>XGELKAIAQELKAIAKELKAIAWEH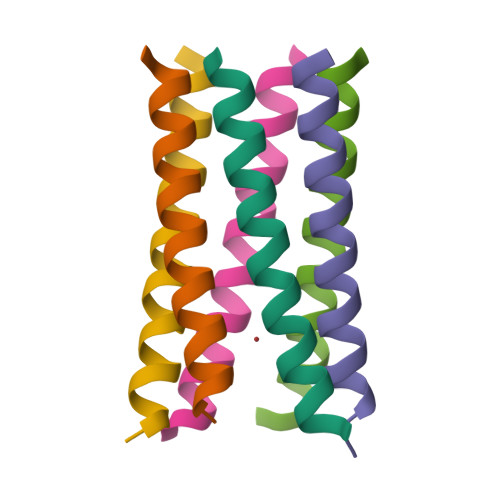KAIAQGAGX[12x]>MSDGTDQSDSGNAVQSAARVERAADGPGGSGGGGSGGGGVGVSTGSYDNQTHYKFLGDGWVEITAYSTRMVHLNMPKSENYCRVRVHNTNDTGTASHMAMDDAHEQIWTPWSLVDANAWGVWFQPSDWQYISNNMIHINLHSLDQELFNVVIKTVTEQNTGAEAIKVYNNDLTAAMMVALDSNNILPYTPAIDNQETLGFYPWKPTIPSPYRYYFSCDRNLSVTYKDEAGTITDTMGLASGLNSQFFTIENTQRINLLRTGDEYATGTYYFDTEPIRLTHTWQTNRHLGQPPQITELPSSDTANATLTARGYRSGLTQIQGRNDVTEATRVRPAQVGFCQPHDNFETSRAGPFKVPVVPADITQGLDHDANGSLRYTYDKQHGQSWASQNNKDRYTWDAVNYDSGRWTNNCFIQSVPFTSEPNANQILTN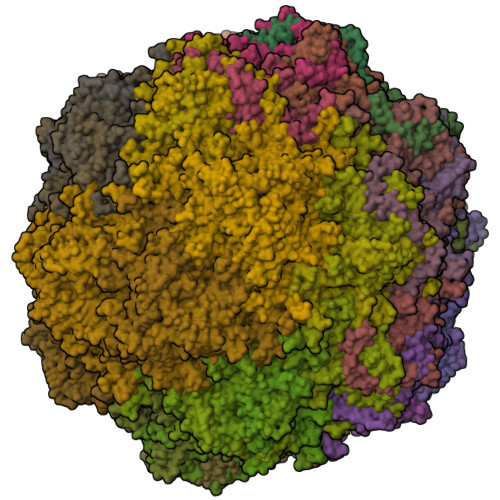RDNLAGKTDIHFTNAFNSYGPLTAFPHPAPIYPQGQIWDKELDLEHKPRLHTQAPFVCKNNAPGQLLVRLAPNLTDQYDPNSSNLSRIVTYGTFFWKGKLTLKAKMRPNATWNPVFQISATNQGTNDYMSIERWLPTATGNITNVPLLSRPVARNTY[60x]> MWLFFGITGLLTAALSGHPSPAPPDQLNTSSAESELWEPGERLPVRLTNGSSSCSGTVEVRLEASWEPACGALWDSRAAEAVCRALGCGGAEAASQLAPPTPELPPPPAAGNTSVAANATLAGAPALLCSGAEWRLCEVVEHACRSDGRRARVTCAENR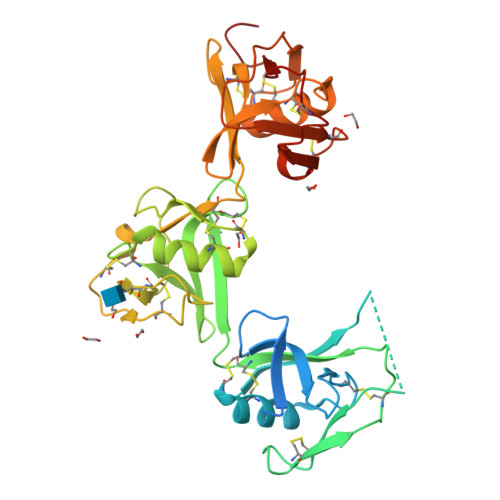ALRLVDGGGACAGRVEMLEHGEWGSVCDDTWDLEDAHVVCRQLGCGWAVQALPGLHFTPGRGPIHRDQVNCSGAEAYLWDCPGLPGQHYCGHKEDAGVVCSEHQSWRLTGGADRCEGQVEVHFRGVWNTVCDSEWYPSEAKVLCQSLGCGTAVERPKGLPHSLSGRMYYSCNGEELTLSNCSWRFNNSNLCSQSLAARVLCSASRGHHHHHH>[2x]MKKIITLFGACALAFSMANADVNLYGPGGPHTALKDIANKYSEKTGVKVNVNFGPQATWFEKAKKDADILFGASDQSALAIASDFGKDFNVSKIKPLYFREAII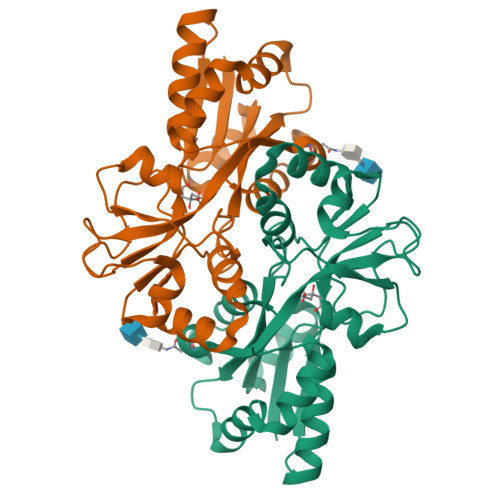LTQKGNPLKIKGLKDLANKKVRIVVPEGAGESNTSGTGVWEDMIGRTQDIKTIQNFRNNIVAFVPNSGSARKLFAQDQADAWITWIDWSKSNPDIGTAVAIEKDLVVYRTFNVIAKEGASKETQDFIAYLSSKEAKEIFKKYGWREH>MGSLDTNPTAFSAFPAGEGETFQPLNADDVRSYLHKAVDFISDYYKSVESMPVLPNVKPGYLQDELRASPPTYSAPFDVTMKELRSSVVPGMTHWASPNFFAFFPSTNSAAAIAGDLIASAMNTVGFTWQASPAATEMEVLALDWLAQMLNLPTSFMNRTGEGRGTGGGVILGTTSEAMLVTLVAARDAALRRSGSDGVAGLHRLAVYAADQTHSTFFKACRLAGFDPANIRSIPTGAETDYGLDPARLLEAMQADADAGLVPTYVCATVGTTSSNAVDPVGAVADVAARFAAWVHVDAAYAGSACICPEFRHHLDGVERVDSISMSPHKWLMTCLDCTCLYVRDTHRLTGSLETNPEYLKNHASDSGEVTDLKDMQVGVGRRFRGLKLWMVMRTYGVAKLQEHIRSDVAMAKVFEDLVRGDDRFEVVVPRNFALV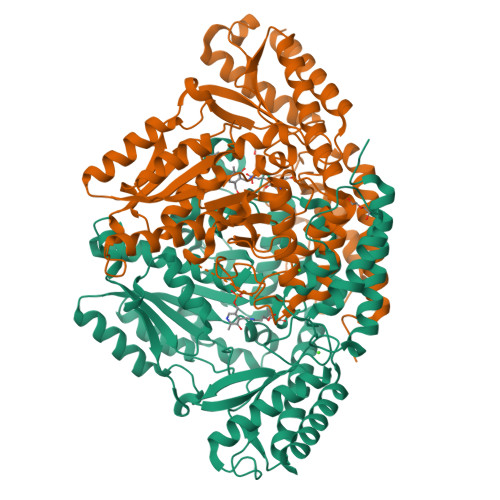CFRIRAGAGAAAATEEDADEANRELMERLNKTGKAYVAHTVVGGRFVLRFAVGSSLQEEHHVRSAWELIKKTTTEMMN[2x]>[4x]GMPHHQYVLTLSCP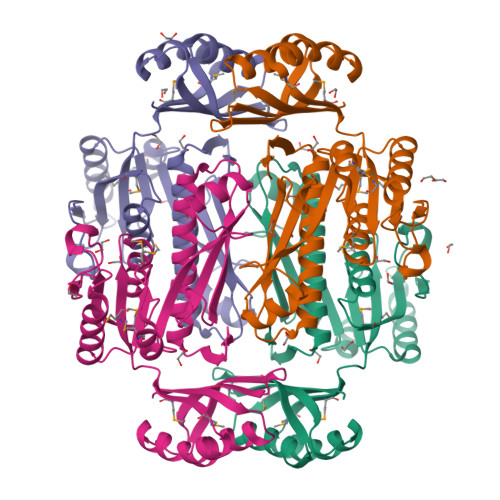DRAGIVSAVSTFLFENGQNILDAQQYNDTESGHFFMRVVFNAAAKVIPLASLRTGFGVIAAKFTMGWHMRDRETRRKVMLLVSQSDHCLADILYRWRVGDLHMIPTAIVSNHPRETFSGFDFGDIPFYHFPVNKDTRRQQEAAITALIAQTHTDLVVLARYMQILSDEMSARLAGRCINIHHSFLPGFKGAKPYHQAFDRGVKLIGATAHYVTSALDEGPIIDQDVERISHRDTPADLVRKGRDIERRVLSRALHYHLDDRVILNGRKTVVFTD> GCGCGUAGUAGC;>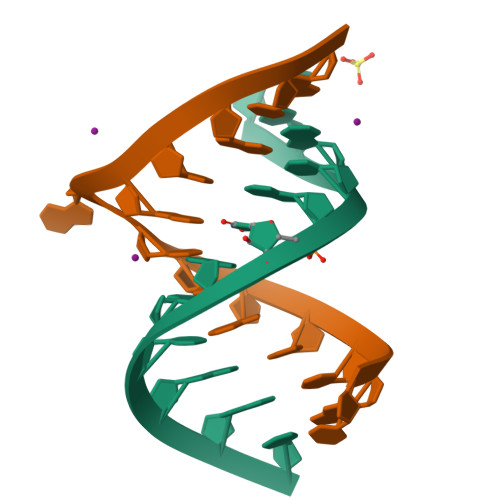 CGCUACUAACGCG> MAHHHHHHMVNAYEVLKEHHVVIKGLGRKISEAPVNSEERHALFDELLIELDIHFRIEDDLYYPALSAATKLIAVAHAEHRQVIDQLSVLLRTPQSE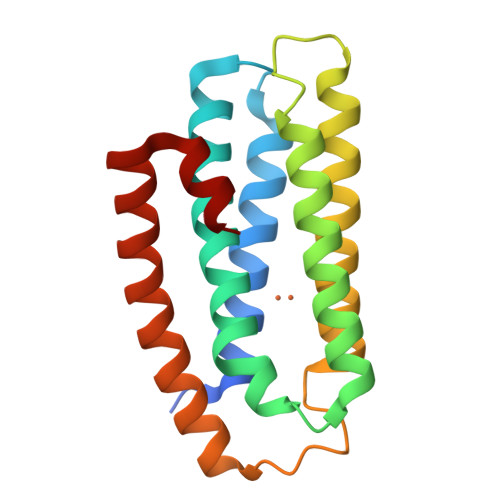PGYEDEWNSFKTVLEAHADEEERDMIPAPPEVKITDAELEELGEKMAARMEQYRGSALYKLRTKGRAALVRSL> SNAMKYTVYLFDFDYTLADSSRGIVTCFRSVLERHGYTGITDDMIKRTIGKTLEESFSILTGITDADQLESFRQEYSKEADIYMNANTILFPD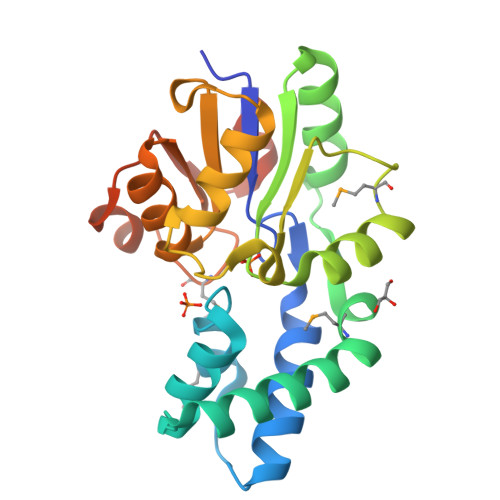TLPTLTHLKKQGIRIGIISTKYRFRILSFLRNHMPDDWFDIIIGGEDVTHHKPDPEGLLLAIDRLKACPEEVLYIGDSTVDAGTAAAAGVSFTGVTSGMTTAQEFQAYPYDRIISTLGQLISVPEDKSGCPL> 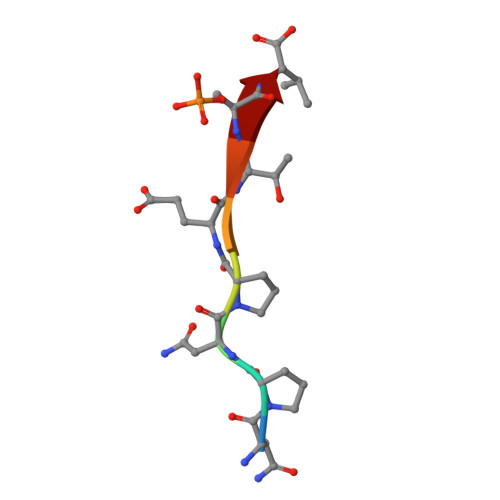NPNPETSV> MNGQHPRSVVTAPDATTGTTSYDVVVVGAGIAGLYAIHRFRSQGLTVR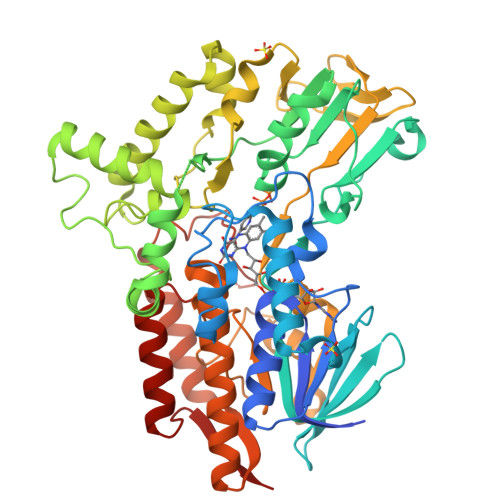AFEAASGVGGVWYWNRYPGARCDVESIDYSYSFSPELEQEWNWSEKYATQPEILAYLEHVADRFDLRRDIRFDTRVTSAVLDEEGLRWTVRTDRGDEVSARFLVVAAGPLSNANTPAFDGLDRFTGDIVHTARWPHDGVDFTGKRVGVIGTGSSGIQSIPIIAEQAEQLFVFQRSANYSIPAGNVPLDDATRAEQKANYAERRRLSRESGGGSPHRPHPKSALEVSEEERRAVYEERWKLGGVLFSKAFPDQLTDPAANDTARAFWEEKIRAVVDDPAVAELLTPKDHAIGAKRIVLDSGYYETYNRDNVELVDLRSTPIVGMDETGIVTTGAHYDLDMIVLATGFDAMTGSLDKLEIVGRGGRTLKETWAAGPRTYLGLGIDGFPNFFNLTGPGSPSVLANMVLHSELHVDWVADAIAYLDARGAAGIEGTPEAVADWVEECRNRAEASLLNSANSWYLGANIPGRPRVFMPFLGGFGVYREIITEVAESGYKGFAILEG> EKEEAIFRSAEMALVQFYIPQEISRDSAYTLGQLGLVQFRDLNSKVRAFQRTFVNEIRRLDNVERQYRYFYSLLKKHDIKLYEGDTDKYLDGSGELYVPPSGSVIDDYVRNASYLEERLIQMEDATDQIEVQKNDLEQYRFILQSGDEFFLKGDNTDSTSYMDEDMIDANGENIAAAIGASVNYVTGVIARDKVATLEQILWRVLRGNLFFKTVEIEQPVYDVKTREYKHKNAFIVFSHGDLIIKRIRKIAESLDANLYDVDSSNEGRSQQLAKVNKNLSDLYTVLKTTSTTLESELYAIAKELDSWFQDVTREKAIFEILNKSNYDTNRKILIAEGWIPRDELATLQARLGEMIARLGIDVPSIIQVLDTNHTPPTFHRTNKFTAGF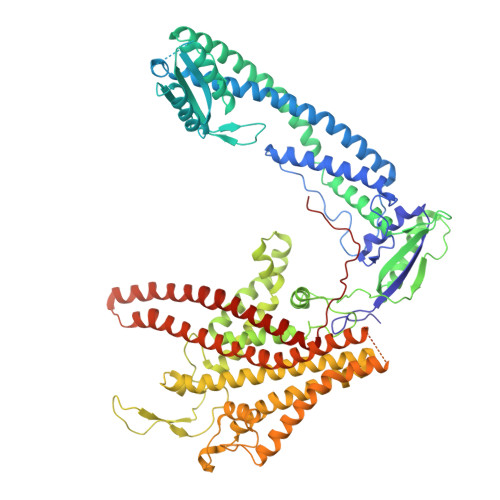QSICDCYGIAQYREINAGLPTIVTFPFMFAIMFGDMGHGFLMTLAALSLVLNEKKINKMKRGEIFDMAFTGRYIILLMGVFSMYTGFLYNDIFSKTMTIFKSGWKWPDHWKKGESITATSVGTYPIGLDWAWHGTENALLFSNSYKMKLSILMGFIHMTYSYFFSLANHLYFNSMIDIIGNFIPGLLFMQGIFGYLSVCIVYKWAVDWVKDGKPAPGLLNMLINMFLSPGTIDDELYPHQAKVQVFLLLMALVCIPWLLLVKPLHFKFTHKKKSHEPLPSTEADASSEDLEAQQLISAMDADDAEEEEVGSGSHGEDFGDIMIHQVIHTIEFCLNCVSHTASYLRLWALSLAHAQLSSVLWTMTIQIAFGFRGFVGVFMTVALFAMWFALTCAVLVLMEGTSAMLHSLRLHWVESMSKFFVGEGLPYEPFAFEYKDM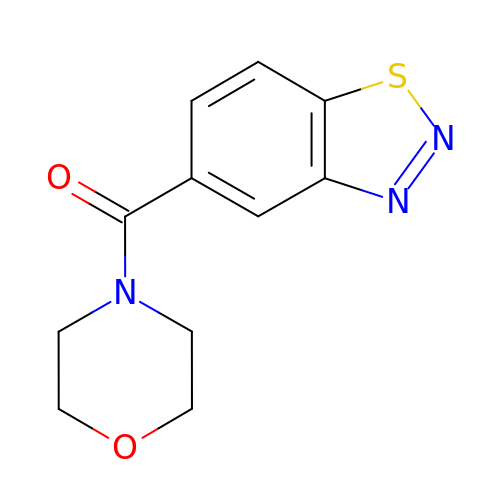(4,7-dihydro-2H-1lambda~4~,2,3-benzothiadiazol-5-yl)(morpholin-4-yl)methanone | C11 H11 N3 O2 S | NDUBYKRNILHJSF-UHFFFAOYSA-N2-{4-chloro-2-[(3-chloro-5-cyanophenyl)carbonyl]phenoxy}-N-(2-methyl-4-sulfamoylphenyl)acetamide | 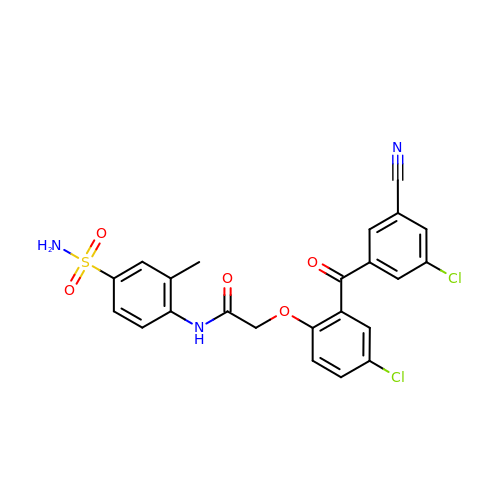C23 H17 Cl2 N3 O5 S | BTOMIMSUTLPSHA-UHFFFAOYSA-N>GLASLADFPIGVAVAASGGNADIFTSSARQNIVRAEFNQITAENIMKMSYMYSGSNFSFTNSDRLVSWAAQNGQTVHGHALVWHPSYQLPNWASDSNANFRQDFARHIDTVAAHFAGQVKSWDVVNEALFDSADDPDGRGSANGYRQSVFYRQFGGPEYIDEAFRRARAADPTAELYYNDFNTEENGAKTTALVNLVQRLLNNGVPIDGVGFQMHVMNDYPSIANIRQAMQKIVALSPTLKIKITELDVRLNNPYDGNSSNDYTNRNDCAVSCAGLDRQKARYKEIVQAYLEVVPPGRRGGIT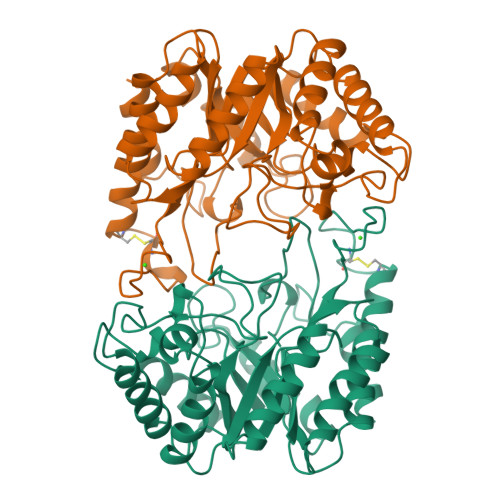VWGIADPDSWLYTHQNLPDWPLLFNDNLQPKPAYQGVVEALSGR[4x]6-{[(3R,4R)-4-{[5-(3-chloro-5-fluorophenyl)pentyl]oxy}pyrrolidin-3-yl]methyl}-4-methylpyridin-2-amine 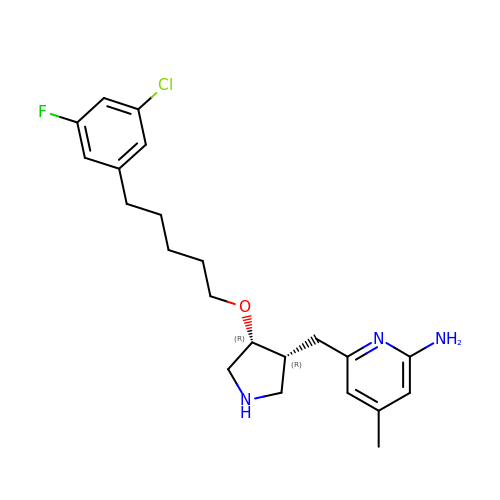| C22 H29 Cl F N3 O | MZDDSPGKIFAODF-UTKZUKDTSA-N> MNQSTSSLVRLASASFAAIGECTSNLARQLFLSSTLTQFRYTTDSVHQPVNEVQSSSTGPASTICGKGDNRTRRGKIFRGTYREQLPSHGPQLHPY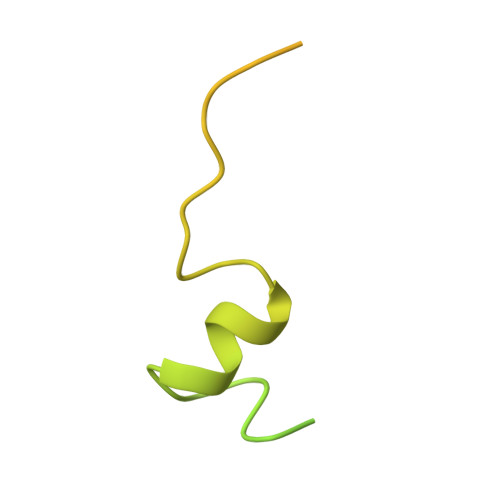PGGPVVQRPGGGSRGAFRYPGEAPPTAPPGASHTVPPAQR> GSMASAAQLRIQKDINELNLPKTCDISFSDPDDLLNFKLVICPDEGFYKSGKFVFSFKVGQGYPHDPPKVKCETMVYHPNIDLEGNVCLNILRE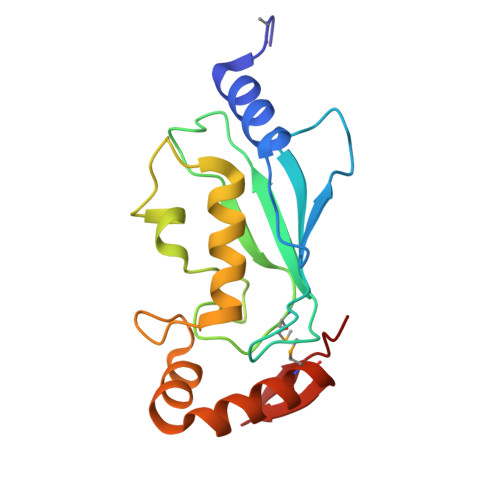DWKPVLTINSIIYGLQYLFLEPNPEDPLNKEAAEVLQNNRRLFEQNVQRSMRGGYIGSTYFERCLK2,1,3-benzothiadiazole-5-carboxylic acid | C7 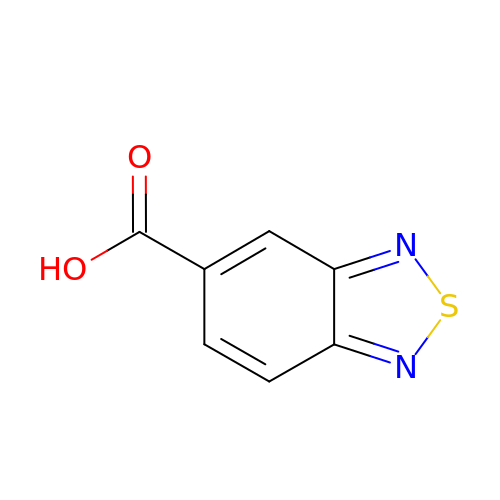H4 N2 O2 S | YHMXJZVGBCACMT-UHFFFAOYSA-N> MWIIEAEGDILKGKSRILFPGTYIVGRNVSDDSSHIQVISKSISKRHARFTILTPSEKDYFTGGPCEFEVKDLDTKFGTKVNEKVVGQNGDSYKEKDLKIQLGKCPFTINAYWRSMCIQFDNPEMLSQWASNLNLLGIPTGLRDSDATTHFVMNRQAGSSITVGTMYAFLK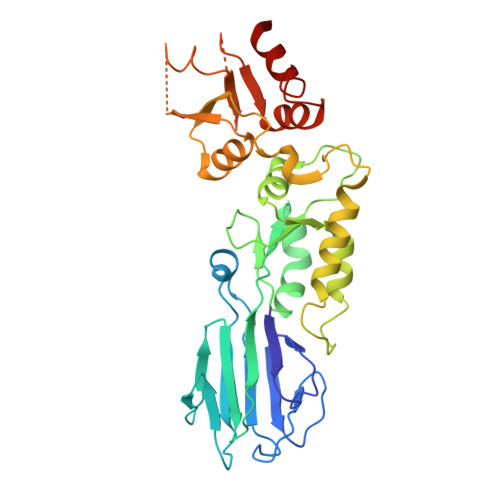KTVIIDDSYLQYLSTVKESVIEDASLMPDALECFKNIIKNNDQFPSSPEDCINSLEGFSCAMLNTSSESHHLLELLGLRISTFMSLGDIDKELISKTDFVVLNNAVYDSEKISFPEGIFCLTIEQLWKIIIERNSRELISKEIERLKYATLVPR>MNLIPTVIETTNRGERAYDIYSRLLKDRIIMLGSQIDDNVANSIVSQLLFLQAQDSEKDIYLYINSPGGSVTAGFAIYDTIQHIKPDVQTICIGMAASMGSFLLAAGAKGKRFALPNAEVMIHQPLGGAQGQATEIEIAANHILKTREKLNRILSERTGQSIEKIQKDTDRDNFLTAEEAKEYGLIDEVMVPETKWSHPQFEK[7x]

In its active tetradecameric conformation, ClpP forms the central proteolytic compartment of a larger AAA+ protease machine. Two rings of seven ClpP monomers stack and interact to form a secluded barrel‐shaped tetradecamer harbouring the 14 catalytic sites. Small entrance pores at the top and bottom of the barrel restrict access of proteins and allow isolated ClpP to degrade small peptides only. For protein degradation, Clp‐ATPases are required (in Firmicutes ClpX, ClpC, and ClpE) to unfold designated substrates and thread them through the entrance pores.

To increase our understanding of the interaction between ADEP and its target in S. aureus, we also determined the crystal structure of ADEP4, a particularly potent ADEP congener, bound to S. aureus ClpP. While typical features of ADEP‐bound ClpP structures from other organisms can also be found here, a specific feature of this SaClpP:ADEP4 structure are the well resolved N‐terminal β‐hairpin loops lining the axial pores. Here, in contrast, residues 4 to 10 and 16 to 20 are well defined in all seven subunits. D27 is in the direct vicinity of the outermost end of the aliphatic tail of ADEP4, corroborating a previous observation of Mabanglo and co‐workers where the corresponding E. coli ClpP residue E40 formed a hydrophobic interaction with the tail of bound ADEP1.33 Binding of ADEP initiates rotations at the key residues of the hydrogen network. The rigidity of the nonpolar side chain of ADEP4 induces a reorientation of the hydrophilic D27 carboxylate, which is the terminal amino acid of helix α1. As illustrated in the enlarged section, this tilt causes a marginal twist of helix α1, thereby shifting the guanidino group of R23 by two angstroms. This generated molecular switch ultimately leads to rearrangements of the unconstrained axial loop stabilising the open gate. When ADEP binds, it stabilises the upwards pointing β‐hairpin conformation. As all ClpP subunits within a ring adopt this up conformation, the pore lumen is no longer blocked. In addition, a subtle but marked outwards movement of the entire N‐terminal domain occurs.>MKMYEVKEFSSGKRKLEDYKSIIGEEEVSKIQEKAEKLKGRSFVHVNSTSFGGGVAEILHSLVPLLRSIGIEARWFVIEGPTEFFNVTKTFHNALQGNESLKLTEEMKELYLNVNRENSKFIDLSSFDYVLVHDPQPAALIEFYEKKSPWLWRCHIDLSSPNREFWEFLRRFVEKYDRYIFHLPEYVQPELDRNKAVIMPPSIDPLSEKNVELKQTEILRILERFDVDPEKPIITQVSRFDPWKGIFDVIEIYRKVKEKIPGVQLLLVGVMAHDDPEGWIYFEKTLRKIGEDYDVKVLTNLIGVHAREVNAFQRASDVILQMSIREGFGLTVTEAMWKGKPVIG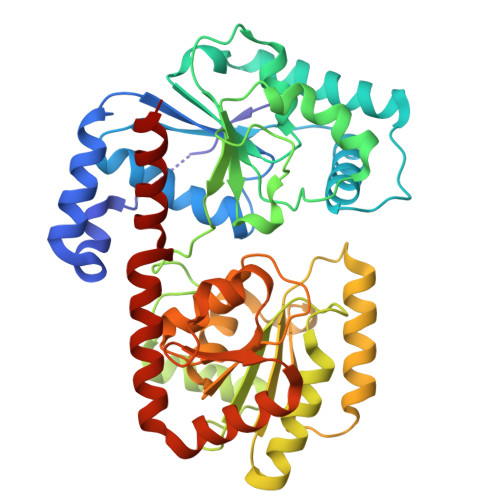RAVGGIKFQIVDGETGFLVRDANEAVEVVLYLLKHPEVSKEMGAKAKERVRKNFIITKHMERYLDILNSLGG[2x]> RDAQRMNILAGRIIAETVRSTLGPKGMDKMLVDDLGDVVVTNDGVTILREMSVEHPAAKMLIEVAKTQEKEVGDGTTTAVVVAGELLRKAEELLDQNVHPTIVVKGYQAAAQKAQELLKTIACEVGAQDKEILTKIAMTSITGKGAEKAKEKLAEIIVEAVSAVVDDEGKVDKDLIKIEKKSGASIDDTELIKGVLVDKERVSAQMPKKVTDAKIALLNCAIEIKETETDAEIRITDPAKLMEFIEQEEKMLKDMVAEIKASGANVLFCQKGIDDLAQHYLAKEGIVAARRVKKSDMEKLAKATGANVITNIKDLSAQDLGDAGLVEERKISGDSMIFVEECKHPKAVTMLIRGTTEHVIEEVARAVDDAVGVVGCTIEDGRIVSGGGSTEVELSMKLREYAEGISGREQLAVRAFADALEVIPRTLAENAGLDAIEILVKVRAAHASNGNKCAGLNVFTGAVEDMCENGVVEPLRVKTQAIQSAAESTEMLLRIDDVIAAEKLR

Chaperonins are homo- or hetero-oligomeric complexes that use ATP binding and hydrolysis to facilitate protein folding. The group II chaperonin from Methanoccocus maripaludis, MmCpn is homo-oligomeric, consisting of two 8-membered rings stacked back-to-back. Chaperonins are further divided into two major subtypes, group I and group II. Both share a similar domain arrangement, in that each subunit consists of three domains: an equatorial ATP-binding domain; an apical domain that is involved in substrate binding; and an intermediate domain that enables communication between the equatorial and apical domains. By contrast, group II chaperonins occur in archaea and eukaryotic cytosol and have a built-in lid segment protruding from the apical domain that opens and closes with ATP binding or hydrolysis.

To further understand the conformational heterogeneity at subunit level, we performed focused classification on each of eight subunits among the ~50% rings from the previous step. We use the same computational procedure to extract and classify the individual single subunit density in each ring. This operation yielded ten classes of distinct subunit conformations. By comparison with published structures of open and closed form of MmCpn with imposed D8 symmetry, we find that these eight well resolved subunit classes covered conformations from the very open all the way to the very closed form. In the difference maps, we find that nucleotide density exists in the four more-closed conformations (class 5–8) but is absent in the four more-open conformations (class 1–4). By freezing the sample immediately after addition of low concentration of ATP, we find that subunits from ~50% of the particles analyzed fall into two major groups, the nucleotide-free open conformation and nucleotide-bound closed conformation. To further test this hypothesis, we reconstructed a map of inter-ring subunit pairs with one subunit in nucleotide-bound closed state (class 8) and the other subunit in nucleotide-unbound open state (class 1), or both subunits in the nucleotide-bound closed state (class 8). We observed little backbone variation at the inter-ring interaction interface as the subunit changed from the open nucleotide-unbound state (class 1) to the nucleotide-bound closed state (class 8). Each subunit conformation can occur in the rings of different nucleotide occupancy. This suggests that conformational change in chaperonin MmCpn is relatively independent in individual subunits of the ring.> AENNLSSQYEEKVRPCIDLIDSLRALGVEQDLALPAIAVIGDQSSGKSSVLEALSGVALPRGSGIVTRCPLVLKLKKLVNEDKWRGKVSYQDYEIEISDASEVEKEINKAQNAIAGEGMGISHELITLEISSRDVPDLTLIDLPGITRVAVGNQPADIGYKIKTLIKKYIQRQETISLVVVPSNVDIATTEALSMAQEVDPEGDRTIGILTKPDLVDKGTEDKVVDVVRNLVFHLKKGYMIVKCRGQQEIQDQLSLSEALQREKIFFENHPYFRDLLEEGKATVPSLAEKLTSELITHISKSLPLLENQIKETHQRITEEL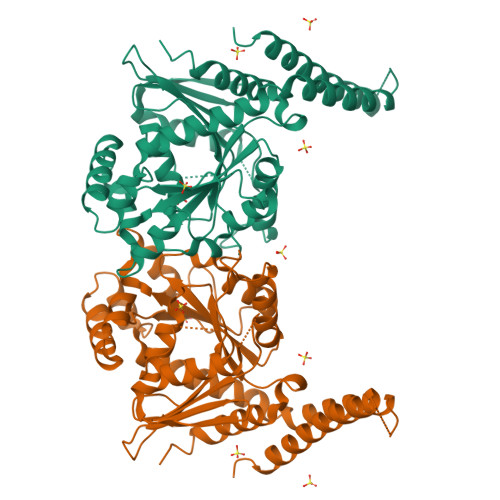QKYGVDIGSGSERSDTSDKRKFLKERLARLTQARRRLAQFPG> GSSPKAVALYSFAGEESGDLPFRKGDVITILKKSDSQNDWWTGRVNGREGIFPANYVEL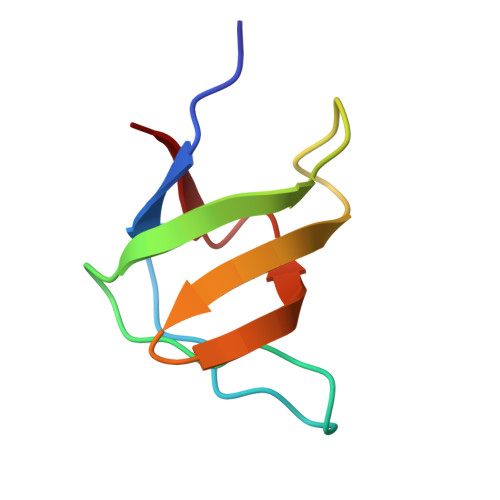V>MTADELVFFVNGKKVVEKNADPETTLLAYLRRKLGLRGTKLGCGEGGCGACTVMLSKYDRLQDKIIHFSANACLAPICTLHHVAVTTVEGIGSTKTRLHPVQERIAKSHGSQCGFCTPGIVMSMYTLLRNQPEPTVEEIEDAFQGNLCRCTGYRPILQGFRTFAKNGGCCGGNGNNPNCCMNQKKDHTVTLSPSLFNPEEFMPLDPTQEPIFPPELLRL[2x];>KDVPPKQLRFEGERVTWIQASTLKELLDLKAQHPEAKLVVGNTEIGIEMKFKNQLFPMIICPAWIPELNAVEHGPEGISFGAACALSSVEKTLLEAVAKLPTQKTEVFRGVLEQLRWFAGKQVKSVASLGGNIITASPISDLNPVFMASGTKLTIVSRGTRRTVPMDHTFFPSYRKTLLGPEEILLSIEIPYSREDEFFSAFKQASRREDDIAKVTCGMRVLFQPGSMQVKELALCYGGMADRTISALKTTQKQLSKFWNEKLLQDVCAGLAEELSLSPDAPGGMIEFRRTLTLSFFFKFYLTVLKKLGKDSKDKCGKLDPTYTSATLLFQKDPPANIQLFQEVPNGQSK[2x];>[2x]EDTVGRPLPHLAAAMQASGEAVYCDDIPRYENELFLRLVTSTRAHAKIKSIDVSEAQKVPGFVCFLSADDIPGSNETGLFNDETVFAKDTVTCVGHIIGAVVADTPEHAERAAHVVKVTYEDLPAIITIEDAIKNNSFYGSELKIEKGDLKKGFSEAD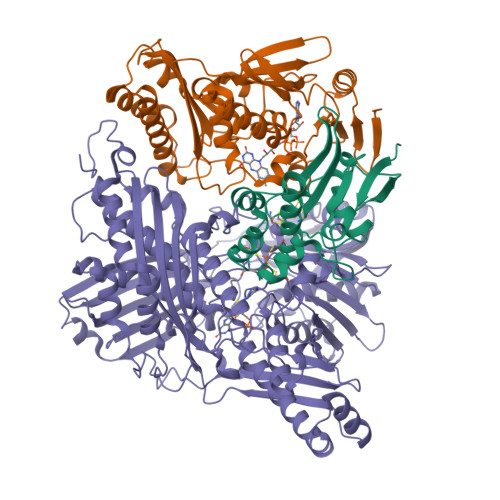NVVSGELYIGGQDHFYLETHCTIAIPKGEEGEMELFVSTQNAMKTQSFVAKMLGVPVNRILVRVKRMGGGFGGKETRSTLVSVAVALAAYKTGHPVRCMLDRNEDMLITGGRHPFLARYKVGFMKTGTIVALEVDHYSNAGNSRDLSHSIMERALFHMDNCYKIPNIRGTGRLCKTNLSSNTAFRGFGGPQALFIAENWMSEVAVTCGLPAEEVRWKNMYKEGDLTHFNQRLEGFSVPRCWDECLKSSQYYARKSEVDKFNKENCWKKRGLCIIPTKFGISFTVPFLNQAGALIHVYTDGSVLVSHGGTEMGQGLHTKMVQVASKALKIPISKIYISETSTNTVPNSSPTAASVSTDIYGQAVYEACQTILKRLEPFKKKNPDGSWEDWVMAAYQDRVSLSTTGFYRTPNLGYSFETNSGNAFHYFTYGVACSEVEIDCLTGDHKNLRTDIVMDVGSSLNPAIDIGQVEGAFVQGLGLFTLEELHYSPEGSLHTRGPSTYKIPAFGSIPTEFRVSLLRDCPNKKAIYASKAVGEPPLFLGASVFFAIKDAIRAARAQHTNNNTKELFRLDSPATPEKIRNACVDKFTTLCVTGAPGNCKPWSLRV>[3x]GAMGSWNPKYDTRTLWTTPDTSPNCTIAQDKDSKLTLVLTKC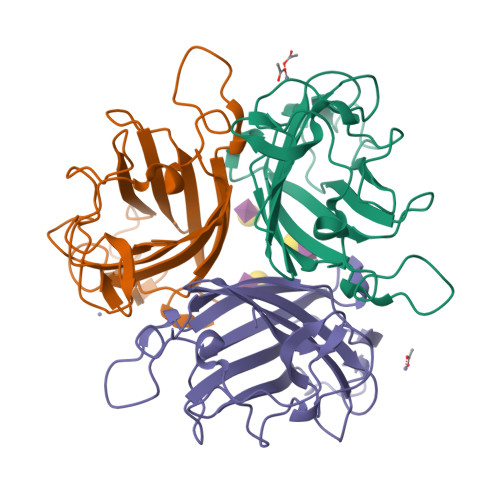GSQILANVSLIVVAGKYHIINNKTNPEIKSFTIKLLFNKNGVLLDNSNLGKAYWNFRSGNSNVSTAYEKAIGFMPNLVAYPKPSNSKKYARDIVYGTIYLGGKPDQPAVIKTTFNQETGCEYSITFDFSWSKTYENVEFETTSFTFSYIAQE3-O-methyl-alpha-D-mannopyranose | C7 H14 O6 | 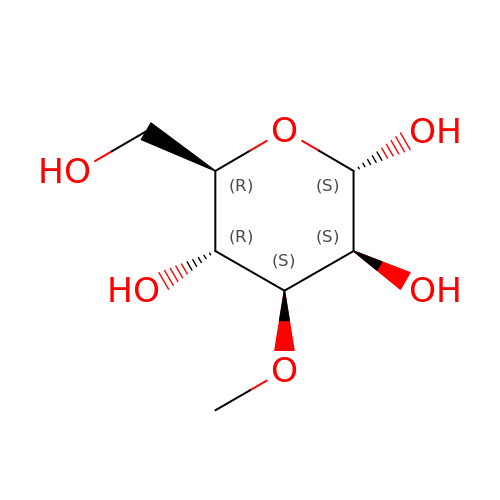SCBBSJMAPKXHAH-VEIUFWFVSA-N> GSARNHTEDNSTEYYDYEEARCACPARHLNNTNGTVLKLLGCHYFCNGTLCTAPDGYPCYNLTAQQVRTLTTYPNTSCAVGVCMKGTCVKNGTMEQCFKTP;> GPSQPKVPEWVNTPSTCCLKYYEKVLPRRLVVGYRKALNCHLPAIIFVTKRNREVCTNPNDDWVQEYIKDPNLPLLPTRNLSTVKIITAKNGQPQLLNSQ

Evasins are chemokine-binding proteins from tick saliva, whose application as anti-inflammatory therapeutics will require manipulation of their chemokine target selectivity. Here we describe subclass A3 evasins, which are unique to the tick genus Amblyomma and distinguished from “classical” class A1 evasins by an additional disulfide bond near the chemokine recognition interface. The A3 evasin EVA-AAM1001 (EVA-A) bound to CC chemokines and inhibited their receptor activation. Structures of chemokine-bound EVA-A revealed a deep hydrophobic pocket, unique to A3 evasins, that interacts with the residue immediately following the CC motif of the chemokine.

To understand how class A3 evasins achieve chemokine binding and inhibition, we purified and crystallised complexes of EVA-A bound to human CCL7, CCL11, CCL16 and CCL17, and solved their structures at resolutions of 1.51–2.01 Å. All four structures display the same fold and 1:1 stoichiometry. In all four chemokine complexes described here, the N-terminus of EVA-A is in contact with the chemokine N-loop. In the EVA-A:chemokine structures, the side chain of the chemokine CC + 1 residue (Tyr in CCL7; Phe in CCL11, Leu in CCL16 and CCL17) sits in a deep hydrophobic pocket within the evasin structure, possibly enabling the ~35° rotation of the chemokine relative to its position in class A1 evasin complexes. To verify the contribution of the CC + 1 residue to affinity, we mutated this residue to Ala in CCL7, CCL11 and CCL16. Surprisingly, CCL16(L19A) exhibited only slightly reduced affinity for EVA-A. Thus, we conclude that the preference of EVA-A for CCL16 over CCL7 and CCL11 is because the aromatic residues in the latter two chemokines are energetically disfavoured, a phenomenon known as negative selection. Here, we found that the preference of EVA-A for chemokines with aliphatic CC + 1 residues results from negative selection against some chemokines with aromatic CC + 1 residues.>[18x]GSHMFTGLNTPHGVAVDSAGTVYVTDHG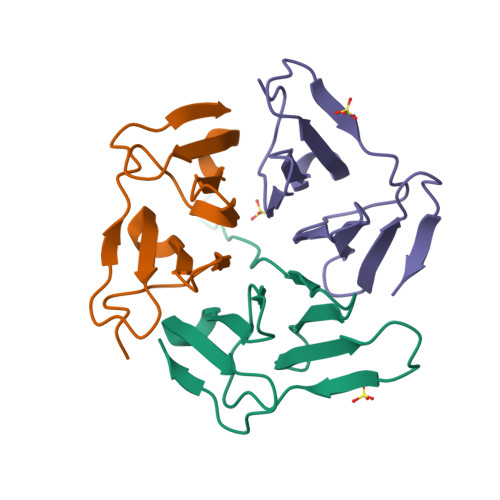NNRVVKLAAGSNTQTVLPFTGLNTPSGVAVDSAGTVYVTDHGNNRVVKLAAGSNTQTVL Originally thought to be redundant but distinct decarboxylases, it has been shown that UbiD is in fact the only decarboxylase, whereas UbiX produces a cofactor strictly required for UbiD activity. The UbiX enzyme catalyses both the N5–C1′ and C6–C3′ bond formation to generate the fourth ring of the prFMN product.

In order to understand the DMAP versus DMAPP preference and any mechanistic consequences, we here determine the crystal structure of the DMAPP-specific Aspergillus niger UbiX (AnUbiX; also called PadA1). We determined the crystal structure of AnUbiX to determine the structural basis of DMAPP versus DMAP specificity. Although AnUbiX was crystallised without any exogenous addition of DMAPP, the crystal structure reveals electron density directly located above the oxidised FMN that corresponds to a bound DMAPP. While the majority of the active-site residues responsible for DMAP(P) binding are conserved in AnUbiX/PaUbiX, a significant variation occurs at position 181 (PaUbiX numbering). In PaUbiX, F181 appears to block binding of a beta-phosphate containing DMAPP in PaUbiX. In comparison, a Gln residue is present in AnUbiX at this position (Q203), establishing a hydrogen bond interaction with the DMAPP beta-phosphate. The crystal structure of the DMAPP-specific AnUbiX reveals a similar interaction between E162 and the DMAPP alpha-phosphate is established, as part of a highly conserved network of polar interaction. We also reveal that the N5 alkylation process occurs when using DMAP in the DMAPP-specific AnUbiX, and is thus independent of the presence of the DMAPP beta-phosphate. However, in this case we show the ensuing Friedel–Crafts alkylation of the flavin C6 only occurs when using DMAPP.

>MFNSLLSGTTTPNSGRASPPASEMPIDNDHVAVARPAPRRRRIVVAMTGATGAMLGIKVLIALRRLNVETHLVMSKWAEATIKYETDYHPSNVRALADYVHNINDMAAPVSSGSFRADGMIVVPCSMKTLAAIHSGFCDDLISRTADVMLKERRRLVLVARETPLSEIHLRNMLEVTRAGAVIFPPVPAFYIKAGSIEDLIDQSVGRMLDLFDLDTGDFERWNGWEK[6x]>[2x]MNAEDVKGFFASRESLDMEQYLVLDYYLESVGDIETALAHFCSEQSTAQWKRVGVDEDFR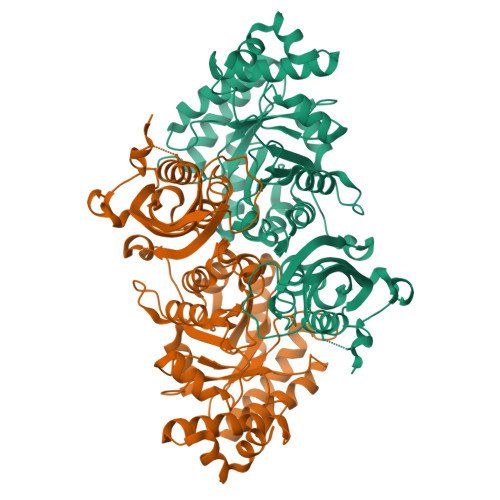LVHAAKVIDYEVIEELEQLSYPVKHSETGKIHACRVTIAHPHCNFGPKIPNLLTAVCGEGTYFTPGVPVVKLMDIHFPDTYLADFEGPKFGIEGLRDILNAHGRPIFFGVVKPNIGLSPGEFAEIAYQSWLGGLDIAKDDEMLADVTWSSIEERAAHLGKARRKAEAETGEPKIYLANITDEVDSLMEKHDVAVRNGANALLINALPVGLSAVRMLSNYTQVPLIGHFPFIASFSRMEKYGIHSKVMTKLQRLAGLDAVIMPGFGDRVMTPEEEVLENVIECTKPMGRIKPCLPVPGGSDSALTLQTVYEKVGNVDFGFVPGRGVFGHPMGPKAGAKSIRQAWEAIEQGISIETWAETHPELQAMVDQSLLKKQD>DVTPRRDAEYPPPEFLEAMKPLREICIKKTGVTEEAIIEFSDGKVHEDENLKCYMNCLFHEAKVVDDTGHVHLEKLHDALPDSMHDIALHMGKRCLYPEGENLCEKAFWLHKCWKESDPKHYFLI[2x]

Odorant-binding proteins (OBPs; aka PBPs, pheromone-binding proteins when they are involved in the detection of pheromones) are the first relay in semiochemical reception in insects as they are the liaison between the air medium that broadcasts chemical signals and odorant receptors, which are located in olfactory structures (mainly the antennae and maxillary palps) of the insect's peripheral sensory system. We studied the structure of the major, female-enriched odorant binding protein (AaegOBP1) from Aedes aegypti, the primary vector for the viruses that cause yellow fever, mostly in tropical regions of Africa and in parts of South America, and human dengue, which infects 100 million people yearly in the tropics and subtropics. Mature AaegOBP1 is a protein with 125 amino acid residues, which shares 82% amino acid identity (91% similarity) with AgamOBP1. The overall structure of AaegOBP1 comprises of six helices (α1 to α6) connected by loops between helices and knitted together by three disulfide bridges between α1 and α3 (C26–C57), helix α3 and the top of helix α6 (C53–C104), and helix α6 and the top of helix α5 (C113–C95).

AaegOBP1 crystallized in space group P21, with unit cell parameters a = 34.37 Å, b = 47.93 Å, c = 69.12 Å and β = 96.50°. Electron density was well defined for most of the structure, except for a few side chains, the first residue of chain A, and the nine initial residues of chain B. The final refined structure contains two monomers of AaegOBP1 with 240 residues, 410 water molecules, 3 Mg2+ ions, one Cl− ion and one putative PEG molecule. Interestingly, the C-terminus is pulled to the core of the protein to form part of the binding pocket wall, which can function as a “lid” for the release of ligands. The C-terminal “lid” is held in place by an array of hydrogen bonds, which is well-conserved between AgamOBP1 and AaegOBP1, namely: Arg5-Asp7, Arg6-Asp42, His121-Asp118, Asp118-Lys120 and Tyr10-Asp7. The carboxylate oxygens of these residues form hydrogen bonds with the hydroxyl of Tyr-54 and the δ-nitrogen of His-23 (AgamOBP1) and Arg-23 (AaegOBP1). It is likely that some of these interactions may be disrupted at low pH leading the C-terminus to move away from the binding cavity thus “opening of the lid” and loosing ligand affinity at low pH. Indeed, AaegOBP1 binds to a mosquito attractant, nonanal, with apparent high affinity at the estimated pH of the sensillar lymph, but with no affinity at the low pH postulated for the environment in the vicinity of odorant receptors due to negative charges surfaces in the neuron membrane. Differences in ligand specificities by these two proteins might be conferred by different residues in the binding cavity, which are located close to the C-terminal lids in AgamOBP1 and AaegOBP1: Leu-15 vs. Phe-15, Leu-19 vs. Met-19, and Ser-79 vs. Ala-79.> DARQFLIYNEDHKRCVDALSAISVQTATCNPEAESQKFRWVSDSQIMSVAFKLCLGVPSKTDWASVTLYAC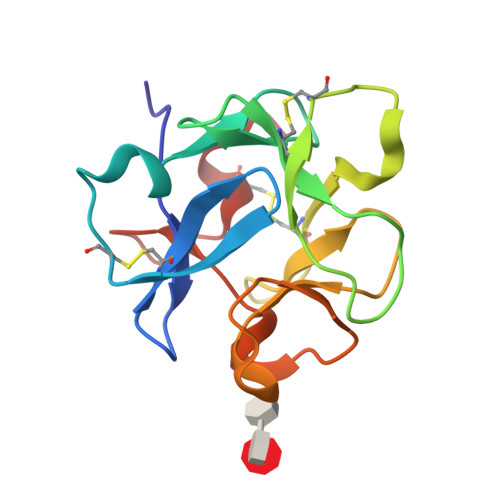DSKSEYQKWECKNDTLFGIKGTELYFNYGNRQEKNIKLYKGSGLWSRWKVYGTTDDLCSRGYE>MSSPYVPTDNRMMQLAYLDRGFYKHYGIIVGESVYQLDSDDIFKTALTGKARFTRTKLTPDWVIEEGCELDYFRVKYLESSVNSEHIFSVDHNCETIAKDIFGTHTLNQHQAIGLVGTILLTAGLMSTIKTPVNATTIKEFFNHAVEGDLEHHHHHH[8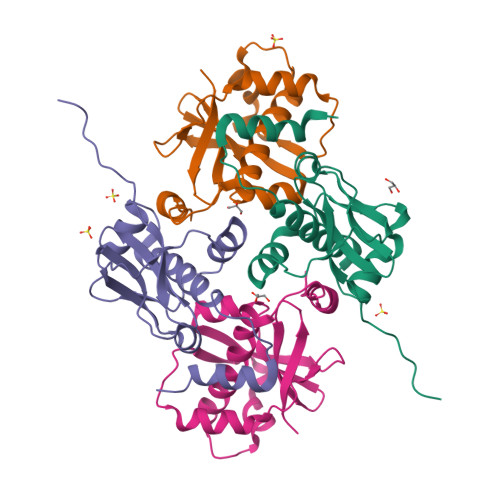x]>[2x]MKSKTLLPAIALLYLTANAQDKRDITAIKNMAGCYEVSFNFSETFSPNKEYKKKDNYHSKALEWVAVVEEQPNKIALQHLLVVNPKGEGKNAIVKHWRQDWLYENTDLYVFNKENHWKYKSLNPKQVKGQWTQIVYQVDDAPRYSGSGTWIHLDEKTFWESTADAPLPRREYTTRTDYNVLNRTNRHEITEWGWLHFQ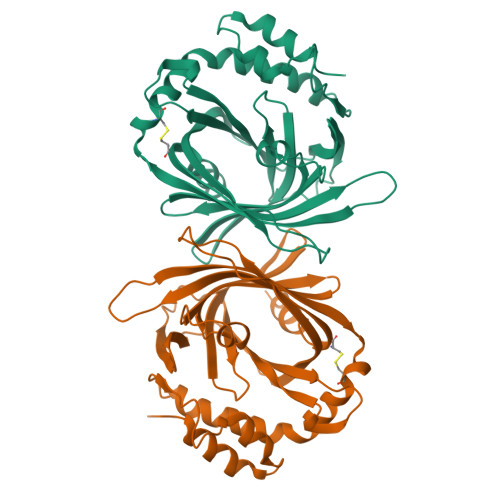DNKKILRQDNQEDTIVAEEIGKEYYKKIDDKKCLIAQNYWKEYAPLWAAVREEWANKMNKKQDLYVKPKVQDTYLYSELMKLEPQQTTEAKELVKKYIVK> RSQGLPGLTVSSPQLRVHVGESVLMGCVVQRTEEKHVDRVDWLFSKDKDDASEYVLFYYSNLSVPTGRFQNRSHLVGDTFHNDGSLLLQDVQKADEGIYTCEIRLKNESMVMKKPVELWVLPEEPRDLRVRVGDTTQMRCSIQSTEEKRVTKVNWMFSSGSHTEEETVLSYDSNMRSGKFQSLGRFRNRVDLTGDISRNDGSI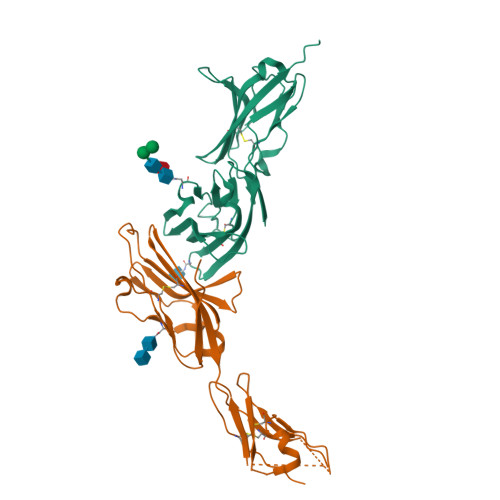KLQTVKESDQGIYTCSIYVGKLESRKTIVLHVVQDEFQRTISPTPPTDKGQQGILNGNQHHHHHH;> SGLSITTPEQRIEKAKGETAYLPCKFTLSPEDQGPLDIEWLISPSDNQIVDQVIILYSGDKIYDNYYPDLKGRVHFTSNDVKSGDASINVTNLQLSDIGTYQCKVKKAPGVANKKFLLTVLVKPSGTRCFVDGSEEIGNDFKLKCEPKEGSLPLQFEWQKLSDSQTMPTPWLAEMTSPVISVKNASSEYSGTYSCTVQNRVGSDQCMLRLDVVPPSNRAHHHHHH>GSHMSNNQTVLPFDGLNYPEGLAVDTQGAVYVADRGNNRVVKLAAGSKTQTVLPFTGLNDPDG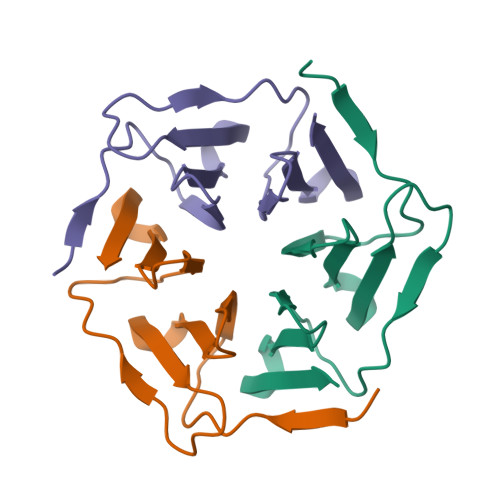VAVDNSGNVYVTDTDNNRVVKLE[3x]N-UNDECANYLPHOSPHONATE METHYL ESTER GROUP | C12 H27 O2 P | 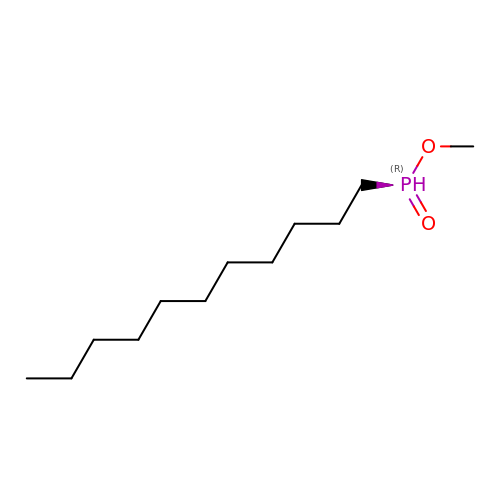FYHIOSOXVZDSJI-UHFFFAOYSA-N> MRGSHHHHHHTDPALRAQDAAPRLTFTLRDEERLMMKIGVFVPIGNNGWLISTHAPQYMPTFELNKAIVQKAEHYHFDFALSMIKLRGFGGKTEFWDHNLESFTLMAGLAAVTSRIQIYATAATLTLPPAIVARMAATIDSISGGRFGVNLVTGW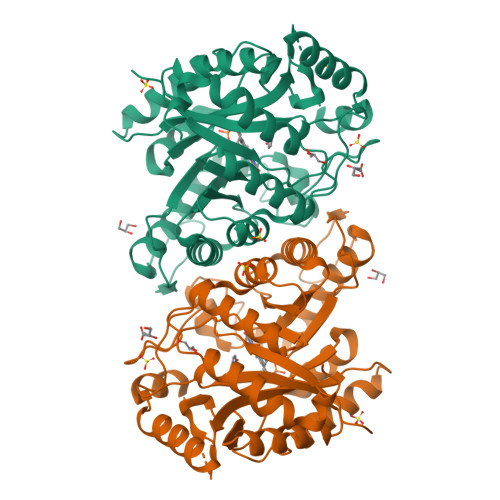QKPEYEQMGIWPGDDYFSRRYDYLTEYVQVLRDLWGTGKSDFKGDFFTMNDCRVSPQPSVPMKVICAGQSDAGMAFSARYADFNFCFGKGVNTPTAFAPTAARMKQAAEQTGRDVGSYVLFMVIADETDDAARAKWEHYKAGADEEALSWLTEQSQKDTRSGTDTNVRQMADPTSAVNINMGTLVGSYASVARMLDEVASVPGAEGVLLTFDDFLSGIETFGERIQPLMQCRAHLPALTQEVAGLCGR> GPHMATGQDRVVALVDMDCFFVQVEQRQNPHLRNKPCAVVQYKSWKGGGIIAVSYEARAFGVTRSMWADDAKKLCPDLLLAQVRESRGKANLTKYREASVEVMEIMSRFAVIERAAIDEAYVDLTSAVQERLQKLQGQPISADLLPSTYIEGLPQGPTTAEETVQKEGMRKQGLFQWLDSLQIDNLTSPDLQLTVGAVIVEEMRAAIERETGFQCSAGISHNKVLAKLACGLNKPNRQTLVSHGSVPQLFSQMPIRKIRSLGGKLGASVIEILGIEYMGELTQFTESQLQSHFGEKNGSWLYAMCRGIEHDPVKPRQLPKTIGCSKNFPGKTALATREQVQWWLLQLAQELE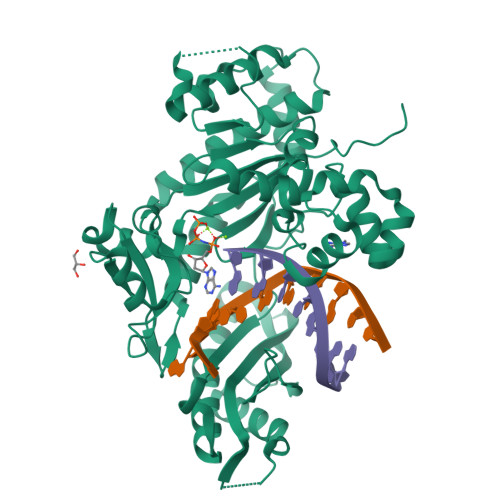ERLTKDRNDNDRVATQLVVSIRVQGDKRLSSLRRCCALTRYDAHKMSHDAFTVIKNCNTSGIQTEWSPPLTMLFLCATKFSAS>[4x]GAAGDGAGASRQRKLEALIRDPRSPINVESLLDGLNSLVLDLDFPALRKNKNIDNFLNRYEKIVKKIRGLQMKAEDYDVVKVIGRGAFGEVQLVRHKASQKVYAM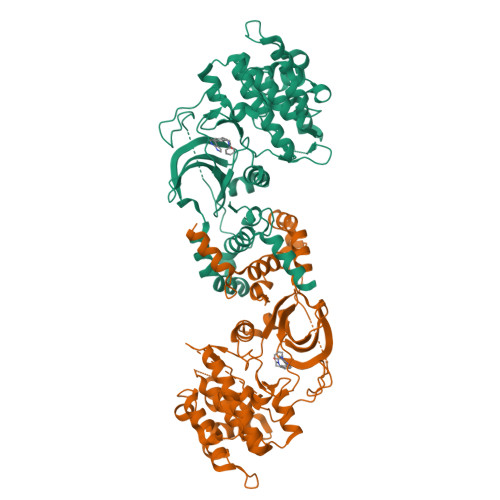KLLSKFEMIKRSDSAFFWEERDIMAFANSPWVVQLFYAFQDDRYLYMVMEYMPGGDLVNLMSNYDVPEKWAKFYTAEVVLALDAIHSMGLIHRDVKPDNMLLDKHGHLKLADFGTCMKMDETGMVHCDTAVGTPDYISPEVLKSQGGDGFYGRECDWWSVGVFLYEMLVGDTPFYADSLVGTYSKIMDHKNSLCFPEDAEISKHAKNLICAFLTDREVRLGRNGVEEIRQHPFFKNDQWHWDNIRETAAPVVPELSSDIDSSNFDDIEDDKGDVETFPIPKAFVGNQLPFIGFTYYR7-{[2-methoxy-4-(1H-pyrazol-4-yl)benzoyl]amino}-2,3,4,5-tetrahydro-1H-3-benzazepinium | C21 H23 N4 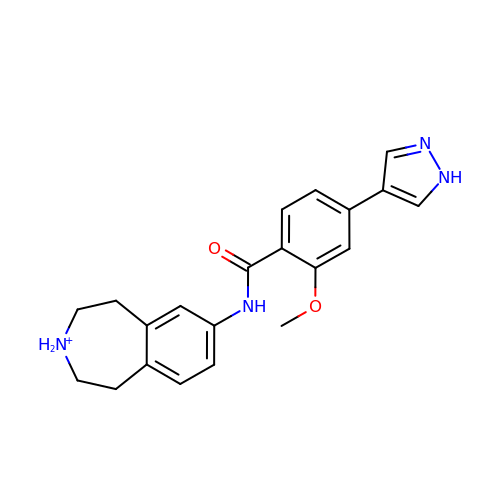O2 | GMZCYCKIXQZORP-UHFFFAOYSA-O> GPGSEFQFPDWIRQFLLGDRGARSGLLQRDEMHAQLQELENKILTKMAEMQGKSAREAAASLGQILQKEGIVGVTEEQVHRIVKQALQRYSEDRIGMVDYALESGGASVISTRCSETYETKTALLSLFG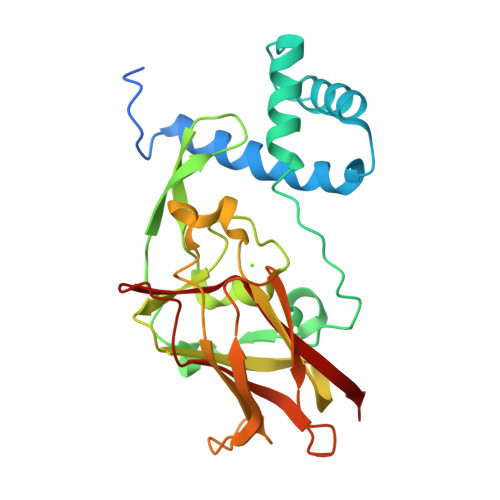IPLWYHSQSPRVILQPDVHPGNCWAFQGPQGFAVVRLSARIRPTAVTLEHVPKALSPNSTISSAPKDFAIFGFDEDLQQEGTLLGTFAYDQDGEPIQTFYFQASKMATYQVVELRILTNWGHPEYTCIYRFRVHGEPAH> SLSSKDKDAVKALWGKIADKAEEIGADA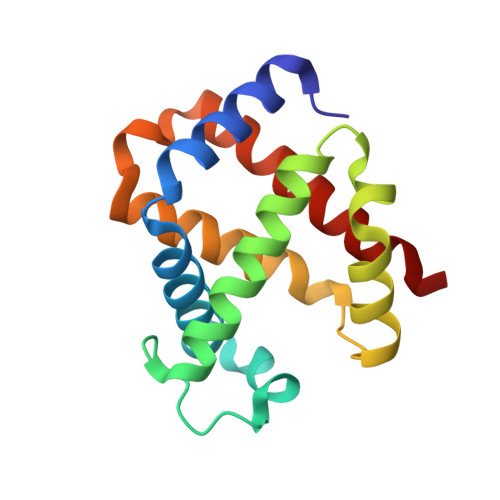LGRMLAVYPQTKTYFSHWKDLSPGSAPVNKHGKTIMGGLVDAVASIDDLNAGLLALSELHAFTLRVDPANFKILSHCILVQLAVKFPKDFTPEVHLSYDKFFSAVARALAEKYR Hypothesizing that a serpin reflecting a highly conserved sequence may offer insight into the delicate balance between folding and function, we designed conserpin (consensus serpin). To design conserpin we used the consensus approach and a previously reported MSA of 219 serpin sequences. Conserpin (396 aa) shares the highest similarity with α1-AT (137 residue differences; 62% sequence identity). Characterization of its function, structure and folding reveal a serpin that is inhibitory, folds reversibly, is thermostable and resistant to polymerisation.

The crystal structure of conserpin, confirms that it adopts the archetypal native serpin fold. Comparison of native and latent state conserpin structures with available native, latent and cleaved structures of α1-AT545556, plasminogen activator inhibitor 1 (PAI-1), α1-antichymotrypsin (ACH), neuroserpin, antithrombin and the thermostable serpins, thermopin63 and tengpin reveal that despite having the highest thermostability, native conserpin has the fewest H-bonds and salt bridges. Further, native state conserpin has the largest accessible surface area and largest solvent inaccessible cavity volume of all assessed serpins. The D-helix of conserpin is shortened by the deletion of five residues, four at the N-terminus (L84, E86, I87 and P88 in α1-AT) and one at the C-terminus (Q109 in α1-AT). The rigidity of hD in conserpin is probably due to a salt bridge between Q105R79 of hD and E376346 and interactions of the N-terminus with hD. Four residues of the extension were resolved in the crystal structure and a single H-bond is observed between the backbone of residue A-1conserpin and the N-terminus of hD (D65conserpin). The breach region, consisting of a highly conserved electrostatic network between residues E342α1-AT, K290α1-AT and D341α1-AT at the top of the A-sheet is important for controlling the conformational change that drives protease inhibition394979. This network is significantly extended in conserpin, compared to α1-AT. Specifically, the mutations of T339E310 and S292K264 contribute to a salt bridge network spanning s3A, s5A and s6A with K191163. Conserpin contains three mutations in this region; Y187A159 and G115A88, which allow s2A to more tightly pack against hF, and Y160W132, which further improves the packing density. Although native conserpin features fewer overall number of polar contacts compared to other metastable serpins, new, specific interactions stabilise a rigidified native state that is less frustrated than α1-AT.

> MHHHHHHENLYFQGAASSHKLAEANTDFAFSLYRELAKSSPDKNIFFSPVSISSALAMLSLGAKGDTHTQILEGLGFNSEADIHQGFQHLLQTLNRPKGLQLKTANGLFVDKSLKLLDSFLEDSKKLYQAEAFSVDFDPEEAKKQINDWVEKQTNGKIKDLLKDLDSDTVLVLVNAIYFKGKWKKPFDPENTKEEDFHVDEKTTVKVPMMSQKGKFYYYHDDELSCKVLELPYKGNASMLIILPDEGGLQHLEQSLTPETLSKWLKSLTRRSVELYLPKFKIEGTYDLKEVLSNLGITDLFSPGADLSGITEEKLYVSKAVHKAVLEVNEEGTEAAAATGVEIVPRSPPEFKADRPFLFLIRENKTGSILFMGKVVNP>[2x]AAVILESIFLKRSQQKKKTSPLNFKKRLFLLTVHKLSYYKYDFERGRRGSKKGSIDVEKITCVETVVPEKNPPPERQIPRRGEESSEMEQISIIERFPYPFQVVYD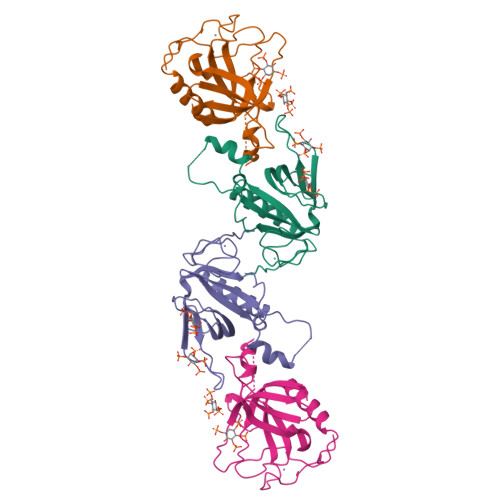EGPLYVFSPTEELRKRWIHQLKNVIRYNSDLVQKYHPCFWIDGQYLCCSQTAKNAMGCQILEN Encapsulins are self-assembling protein nanocompartments capable of selectively encapsulating dedicated cargo proteins, including enzymes involved in iron storage, sulfur metabolism, and stress resistance. Encapsulation is mediated by specific cargo protein motifs known as targeting peptides (TPs), though the structural basis for encapsulation of the largest encapsulin cargo class, dye-decolorizing peroxidases (DyPs), is currently unknown. In this study, we report the structural and functional analysis of a DyP encapsulin system from a Gram-negative pathogen – Klebsiella pneumoniae (Kp). DyPs are ubiquitous, often homohexameric, heme-containing enzymes, named for their ability to oxidize and degrade a wide range of synthetic dyes – with concomitant reduction of hydrogen peroxide to water.

To overcome this challenge, we utilize a heterologous cargo-loading strategy based on a small and monomeric cargo protein (SUMO), fused to the native KpDyP TP, which allowed us to achieve sufficient TP occupancy for cryo-EM analysis of the TP binding site. In particular, the C-terminal 22 residues of KpDyP – containing the putative TP – were fused to the C-terminus of the 11 kDa monomeric small ubiquitin-like modifier (SUMO) protein via an 11-residue flexible glycine-serine linker. After heterologous expression and purification, single-particle cryo-EM analysis was carried out on SUMO-loaded KpEnc (SUMO-TP_Enc). The consensus icosahedral (I) refinement yielded a resolution of 2.4 Å and the resulting cryo-EM density showed substantially improved signal for the KpDyP TP. As such, a ten-residue TP could be confidently modeled (SGSLNIGSLK) highlighting the details of the TP-shell interaction. In particular, TP-shell binding is mediated by a combination of hydrophobic, ionic, and H-bonding interactions. The three hydrophobic residues Leu340, Ile342, and Leu345 of the KpDyP TP interact with a geometrically complementary hydrophobic pocket located on the interior surface of the encapsulin shell protein. Additionally, Lys346 forms a salt bridge with an aspartate side chain carboxyl (Asp38) which is part of the shell protein P-domain. Multiple hydrogen bonds also contribute to TP binding, including interactions between the TP backbone (Leu345 and Gly343) and encapsulin shell residues Arg34 and Asp229. Finally, an intramolecular hydrogen bond between the two TP residues Asn341 and Ser339 appears to stabilize the observed TP conformation.

> MNNLHRELAPVSDAAWEQIEEEASRTLKRFLAARRVVDVSDPQGPAFSAVGTGHVTRLEGPGDSVGAVKRQSQPVVEFRVPFILTRQAIDDVERGSQDSDWSPLKEAARKIAGAEDRAVFDGYAAAGIGGIRPQSSNSPLTLPVAASGYPDVIARALDQLRVAGVNGPYHLVLGENAYTLITSGNEDGYPVLQHIHRLIDGEIVWAPAIEGGVLLSTRGGDFAMDIGQDISIGYLSHTATHVELYLQESFTFRTLTSEAVVSLLPSED;> SGSLNIGSLK>MKKGHHHHHHGSERTGTQPLGVQGLTEEQRMMIRELMDAQMKTFDTTFSHFKNFRLPGVLSSGCELPESLQAPSREEAAKWSQVRKDLCSLKVSLQLRGEDGSVWNYKPPADSGGKEIFSLLPHMADMSTYMFKGIISFAKVISYFRDLPIEDQISLLKGAAFELCQLRFNTVFNAETGTWECGRLSYCLEDTAGGFQQLLLEPMLKFHYMLKKLQLHEEEYVLMQAISLFSPDRPGVLQHRVVDQLQEQFAITLKSYIECNRPQPAHRFLFLKIMAMLTELRSINA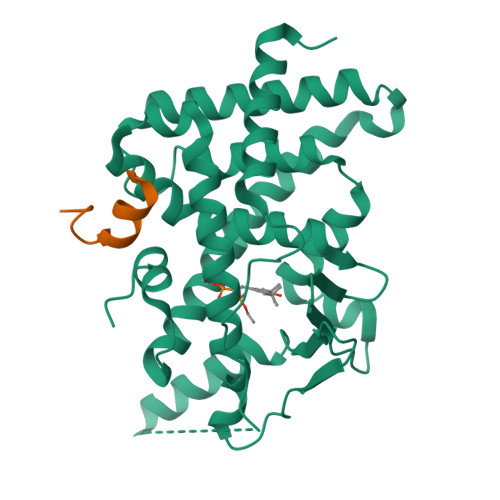QHTQRLLRIQDIHPFATPLMQELFGITGS[2x];>CPSSHSSLTERHKILHRLLQEGSPS[2x]> AEETCFDKYTGNTYRVGDTYERPKDSMIWDCTCIGA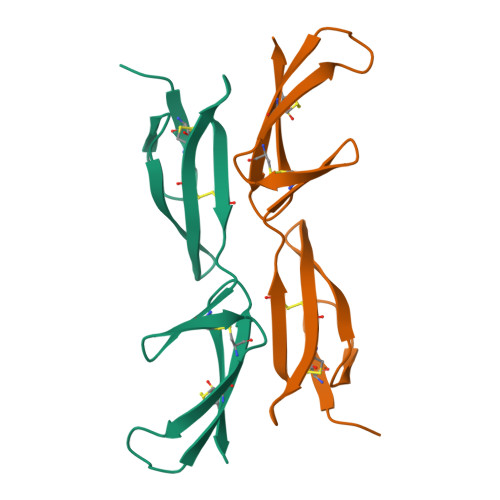GRGRISCTIANRCHEGGQSYKIGDTWRRPHETGGYMLECVCLGNGKGEWTCKPI>MDIAKWVEHARTCYSTQLDTKIKVIGVIGKDYPDHGKGDNINCYLRENVFPVAATEDETCTIRGHFSEDDQILFLVMNGVDDVANIRKCLKSNPKSNYFDAMAESECQQIRMLHFLFISCHFIIIFEQTSRIDLELMRFLKKVNSARIQLRKKINQRLVASDLRDVSFNNRILSSAESEGRMVVPRLLIAFQRNNIRPDVNPGKKLQRELYEKLEKNLDNQFSDILKLYDLIDCGASSLCQLNETIPVVHLLNPKIVKRDIIGEMFEILMADAENTKISGNAGTLPSNNSFVKFLEDNFRSEKNEISLENVIELMNCLQCVLDGDLEEKHEKTAIQTFIKRIQNDHMEEARRLYTNAQRPGERRGADRFKDSEKPVKIRSKEEHLMRFNEATHYIDSVVGVNSREALSQLQAQCNEMWQSDMRHHHHHH[3x];>MKESVRFLTDFGEISDAISDLLTSSPNFNVISAIGPQGAGKSTLLSMLAGNNSRQMYREYVFRPVSREANEQSRHQTIQIDIYIVNHQIFLDCQPMYSFSIMEGLPKVRGGRFDDSTAMSDTLRLTAFLLYVSHTVLVVSETHYDKVIIDTLRVAEQIRPYLAIFRPKLAIDRKTNLVFIKTKASSIDLAPTVIREREELLRLSFQDSRWLKVSQEPFKTLIVLE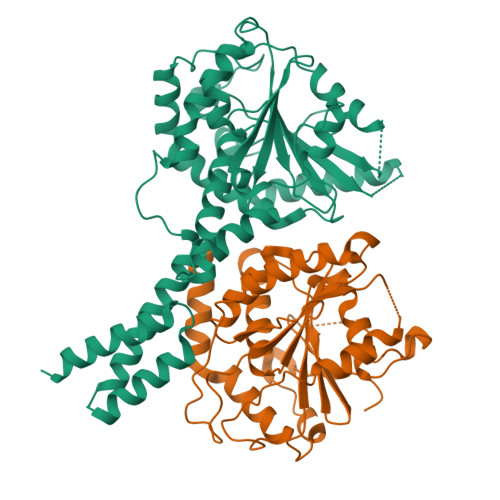EIRVRREHLFEEGDEPDEAASLNEFDEQIAELREELQKNREDFTVETAAMDEKKWLDMCREVIRDKTLHKTLKEYQRAMTDGVRTHFDNGFH[3x]(2~{R},4~{S},6~{S})-4-[2,4-bis(fluoranyl)-5-pyrimidin-5-yl-phenyl]-6-(3,5-dimethyl-1,2-oxazol-4-yl)-1,3-thiazinan-2-amine 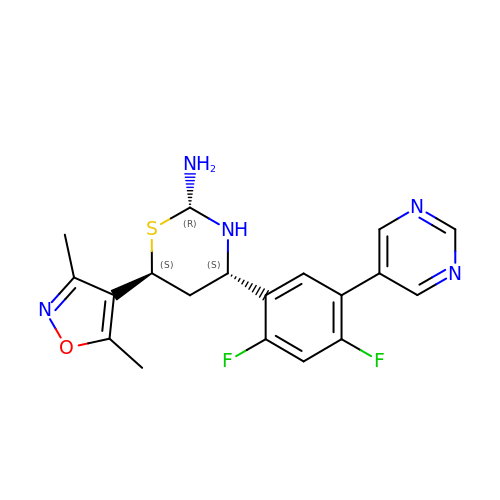| C19 H19 F2 N5 O S | QXXCXVMLHLDXDN-JENIJYKNSA-N(5R)-4-(5-bromofuran-2-carbonyl)-5-(4-fluorophenyl)-7-methyl-1,3,4,5-tetrahydro-2H-1,4-benzodiazepin-2-one 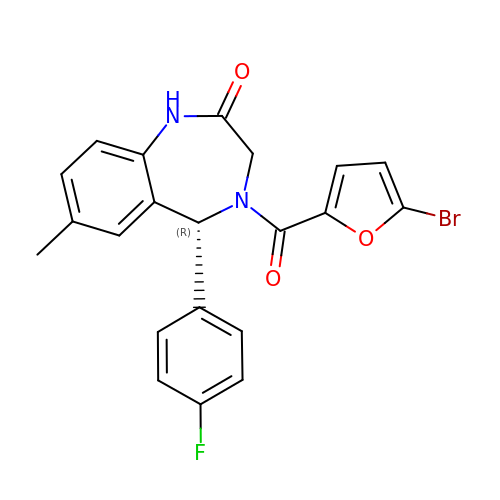| C21 H16 Br F N2 O3 | IPHKQIFYQWJQAB-HXUWFJFHSA-N>DEAAELMQQVNVLKLTVEDLEKERDFYFGKLRNIELICQENEGENDPVLQRIVDILYA[8x];>GSTRRR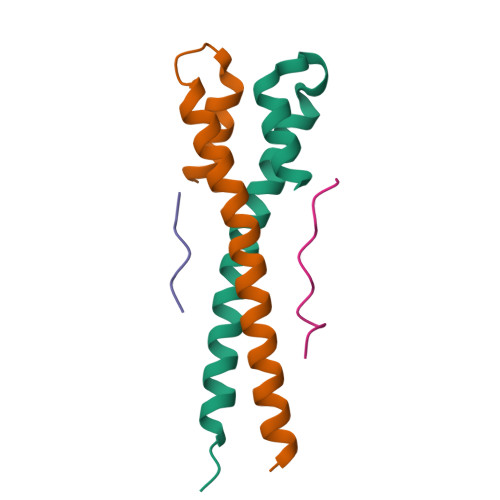TRLRPPTPLSQLLSP[8x]>MTPASYNLAVRRAAPAVVNVYNRGLNTNSHNQLEIRTLGSGVIMDQRGYIITNKHVINDADQIIVALQDGRVFEALLVGSDSLTDLAVLKINATGGLPTIPINARRVPHIGDVVLAIGNPYNLGQTITQGIISATGRIGLNPTGRQNFLQTDASINHGNSGGALVNSLGELMGINTLSFDKSNDGETPEGIGFAIPFQLATKIMDKLIRDGRVIRGYIGIGGREIAPLHAQGGGIDQLQGIVVNEVSPDGPAANAGIQVNDLIISVDNKPAISALETMDQVAEIRPGSVIPVVVMRDDKQLTLQVTIQEY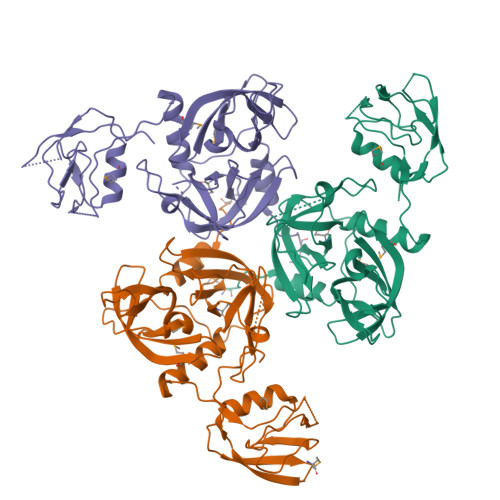PATNHHHHHH[3x]>[12x]MAQDIFLKIDGINGESLDDSHKDEIEVLNWNWEIQQESTMHTGSGGGAGKASVK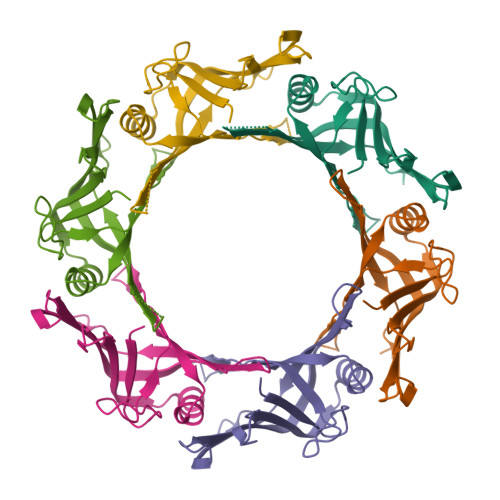DLTFEHAIDRASPNLMKYALTGKHVDQAVLVMRKAGGNPLEYLKLTMSDVIITRVRPSGSRDDTERSRETVSLSFAKVKQEYVVQNAQGGSGGAVTTSFDIKGNKEA>MKEEKRSSTGFLVKQRAFLKLYMITMTEQERLYGLKLLKVLQSEFKEIGFKPNHTEVYRSLHELLDDGILKQIKV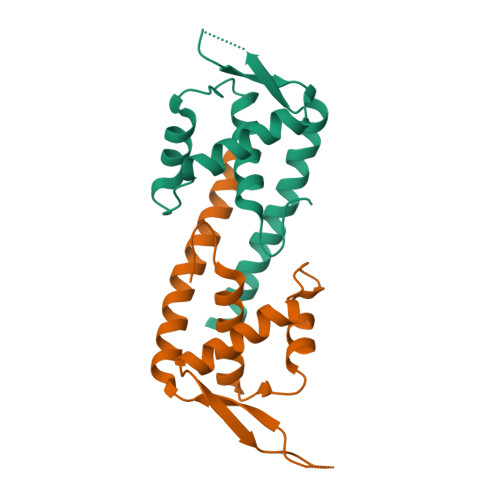KKEGAKLQEVVLYQFKDYEAAKLYKKQLKVELDRCKKLIEKALSDNF[4x]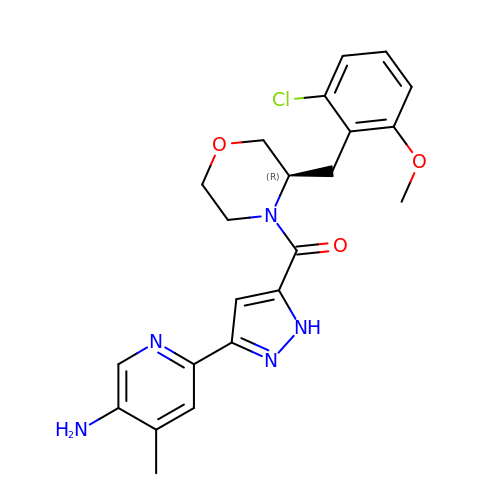[3-(5-amino-4-methylpyridin-2-yl)-1H-pyrazol-5-yl]{(3R)-3-[(2-chloro-6-methoxyphenyl)methyl]morpholin-4-yl}methanone | C22 H24 Cl N5 O3 | ZAPLCZOOCDRDCZ-CQSZACIVSA-N> GSHMGLTFNSNNICIDDNINTLWTGVNPTTANCQIMASSESNDCKLILTLVKTGALVTAFVYVIGVSNDFNMLTTHKNINFTAELFFD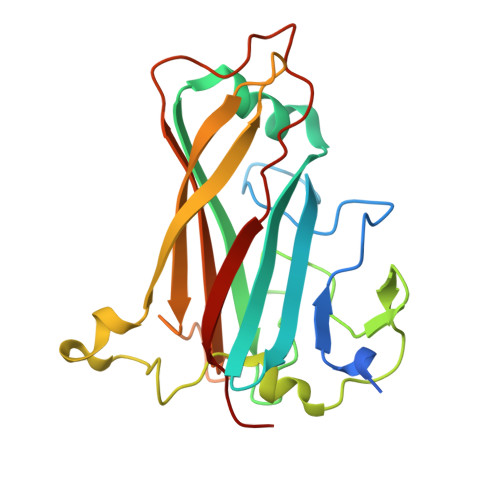STGNLLTSLSSLKTPLNHKSGQNMATGALTNAKGFMPSTTAYPFNVNSREKENYIYGTCYYTASDHTAFPIDISVMLNQRALNNETSYCIRVTWSWNTGVAPEVQTSATTLVTSPFTFYYIREDD N-HYDROXYUREA | C H4 N2 O2 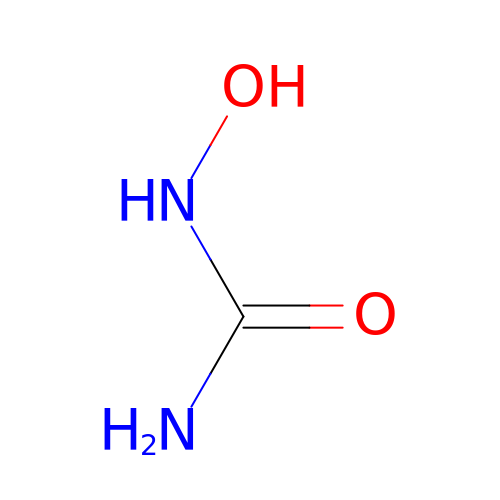| VSNHCAURESNICA-UHFFFAOYSA-N> MGKEKSHINVVVIGHVDSGKSTTTGHLIYKCGGIDKRTIEKFEKEAAELGKGSFKYAWVLDKLKAERERGITIDIALWKFETPKYQVTVIDAPGHRDFIKNMITGTSQADCAILIIAGGVGEFEAGISKDGQTREHALLAFTLGVRQLIVAVNKMDSVKWD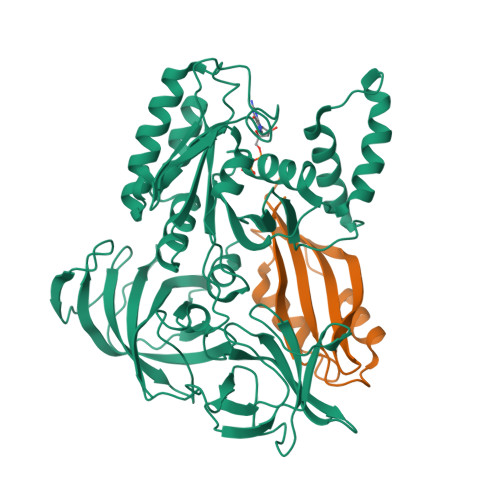ESRFQEIVKETSNFIKKVGYNPKTVPFVPISGWNGDNMIEATTNAPWYKGWEKETKAGVVKGKTLLEAIDAIEQPSRPTDKPLRLPLQDVYKIGGIGTVPVGRVETGVIKPGMVVTFAPAGVTTEVKSVEMHHEQLEQGVPGDNVGFNVKNVSVKEIRRGNVCGDAKNDPPKGCASFNATVIVLNHPGQISAGYSPVLDCHTAHIACRFDELLEKNDRRSGKKLEDHPKFLKSGDAALVKFVPSKPMCVEAFSEYPPLGRFAVRDMRQTVAVGVIKSVDKTEKAAKVTKAAQKAAKK;> KPAKPAAKSIVTLDVKPWDDETNLEEMVANVKAIEMEGLTWGAHQFIPIGFGIKKLQINCVVEDDKVSLDDLQQSIEEDEDHVQSTDIAAMQAL>[6x]GPGYQMESNGVPMITLSSGIRMPALGMGTAETMVKGTEREKLAFLKAIEVGYRHFDTAAAYQSEECLGEAIAEALQLGLIKSRDELFITSKLWCADAHADLVLPALQNSLRNLKLDYLDLYLIHHPVSLKPGKFVNEIPKDHILPMDYKSVWAAMEECQTLGFTRAIGVCNFSCKKLQELMAAAKIPPVVNQVEMSPTLHQKNLREYCKANNIMITAHSVLGAICAPWGSNAVMDSKVLHQIAVARGKSVAQVSMRWVYQQGASLVVKSFNEGRMKENLKIFDWELTAENMEKISEIPQSRTSSADFLLSPTGPFKTEEEFWDEKD

The aldo-keto reductase (AKR) codeinone reductase (COR) catalyzes the final and penultimate steps in the biosynthesis of codeine and morphine, respectively, in opium poppy (Papaver somniferum). COR belongs to the large and well-studied AKR superfamily, which is characterized by the TIM-barrel fold and mechanistically flexible NAD(P)H dependant oxidoreductase activity. The overall three-dimensional structure of COR reveals a TIM-barrel fold common to the AKR superfamily, in which eight parallel β-strands form a central barrel surrounded by eight α-helices to form the (α/β)8 barrel. The residues that form the canonical catalytic tetrad are contributed by the β2α2 loop (Asp-51 and Tyr-56), β3 (Lys-86) and loop A (His-119).

The crystal structure of the COR1.3 isoform (hereafter referred to as COR) was solved using molecular replacement and refined to a resolution of 2.4 Å. Although 1 mM NADPH and 1 mM codeine were present during crystallization, no electron density corresponding to NADPH was seen. Although weak electron density was seen in the active site at a location expected for codeine, this electron density was too weak to define a precise mode of binding. The crystal structure described in this paper thus represents an apoenzyme state with a well-defined binding pocket for the NADPH cofactor similar to that seen for other AKRs binding to either NADPH or NADH. The most notable structural feature of COR is the shifting of the β1α1 loop away from the cofactor binding tunnel, which is made particularly evident when compared with structures of CHR and 3α-HSD. The distinctive conformation adopted by the β1α1 loop widens the cofactor binding tunnel and helps to define the putative binding site for the alkaloid substrate, primarily through the side chain and carbonyl group of Glu-26 and the side chain of Met-28. The asymmetric unit of this crystal structure of apo-COR reveals three homodimers with C2 rotational symmetry. A single disulfide bond is formed between Cys-220 of each protomer near the bottom of the V-shaped cleft. The lack of conservation of the Cys-220 residue and the reported localization of COR in a reducing environment in the plant suggest that the intermolecular disulfide bond may be the result of purifying and crystallizing COR in an aerobic environment, even though reducing agent was present during purification, and protein samples were stored at –80 °C prior to crystallization.During LPS biosynthesis, a membrane-associated glycosyltransferase (LpxB) forms a tetra-acylated disaccharide that is further acylated to form the membrane anchor moiety of LPS. LpxB is a glycosyltransferase in the Raetz (lipid A synthesis) pathway that catalyzes nucleophilic attack of the 6′-hydroxyl of lipid X (1) on the anomeric carbon of UDP-diacyl-glucosamine (UDP-DAG) (2) to form β(1–6)-tetraacyl-disaccharide 1-phosphate (lipid A disaccharide) (3). Here we present the first crystal structures of a soluble variant of E. coli LpxB in the apo form and bound to UDP, which reveals a novel glycosyltransferase-B (GT-B) dimer wherein the C-terminal tail of one subunit completes the fold of the other subunit. The structure reveals that LpxB has a glycosyltransferase-B family fold but with a highly intertwined, C-terminally swapped dimer comprising four domains.

LpxB6S was crystallized with one molecule in the asymmetric unit. However, the biological assembly is a highly intertwined, C-terminally swapped homodimer. Each half of the LpxB dimer consists of two Rossmann-like domains with a parallel β-sheet core sandwiched between α-helices. The first Rossmann-like domain is composed of the N-terminal half of one subunit (residues 1–166) and the last helix (369–382) from the C-terminus of the other subunit. This domain is connected via short antiparallel helical linkers to the second domain, which is composed of residues 177–295 of the first subunit and 296–345 of the second subunit. LpxB forms a two-fold symmetric dimer in which the polypeptide chains crossover at helix 14 around the dyad axis to swap the remainder of the polypeptide chain. The reciprocally swapped C-terminal segments wrap around the opposing subunit in an interlocked arrangement. These extensive interactions bury a total surface area of 12,650 Å2, forming an LpxB dimer with an overall ‘bowtie’-shape. LpxB in our crystal structure appears to be in an open conformation.

> MTEQRPLTIALVAGETSGDILGAGLIRALKEHVPNARFVGVAGPRMQAEGCEAWYEMEELAVMGISESSGRSRRSSHIRADLTKRFGELKPDVFVGIDAPDFNITLEGNLKKQGIKTIHYVSPSVWAWRQKRVFKIGRATDLVLAFLPFEKAFYDKYNVPCRFIGHTMADAMPLDPDKNAARDVLGIPHDAHCLALLPGSRGAEVESLSADFLKTAQLLRQTYPDLEIVVPLVNAKRREQFERIKAEVAPDLSVHLLDGMGREAMVASDAALLASGTAALECMLSKCPMVVGYRMKPFTFWLAKRLVKTDYVSLPNLLAGRELVKELLQEECEPQKLAAALLPLLANGKTSHAMHDTFRELHQQIRCNADEQAAQAVLELAQ>[2x]LKQVRPGMDLSKVVLPTFILEPRSFLDKLSDYYYHADFLSEAALEENPYFRLKKVVKWYLSGFYKKPKGLKKPYNPILGETFRCLWIHPRTNSKTFYIAEQVSHHPPISAFYVSNRKDGFCLSGSILAKSKFYGNSLSAILEGEARLTFLNRGEDYVMTMP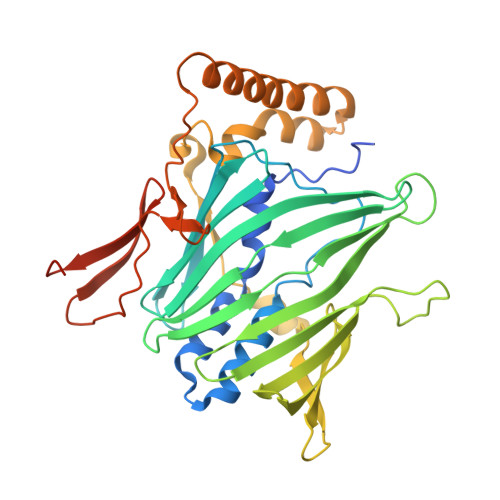YAHCKGILYGTMTLELGGTVNITCQKTGYSAILEFKLKPFLGSSDCVNQISGKLKLGKEVLATLEGHWDSEVFITDKKTDNSEVFWNPTPDIKQWRLIRHTVKFEEQGDFESEKLWQRVTRAINAKDQTEATQEKYVLEEAQRQAARDRKTKNEEWSCKLFELDPLTGEWHYKFADTRPWDPLNDMIQFEKDGVIQTKVKHRTPMVSVPKMKHKPTRQQK>HHHHHHEFFADGKAGLELRNFYFNRDYRQPGASQSYSEEWAQGFLLRYESGYTEGLFGLGVDALGLLGVRLDSSPERSGSGLLPYSTSDRRAAHDYSSLGLTAKLRVSHSTLKIGTLMPRLPVVQFNDTRLHPQTFQGGLLEVNEIDGLALQFGQLRQVKQRDSTNAEDLGITRGNKRNVLAGRHPGSDRFDFAGGTYRWSERLSSSYHYA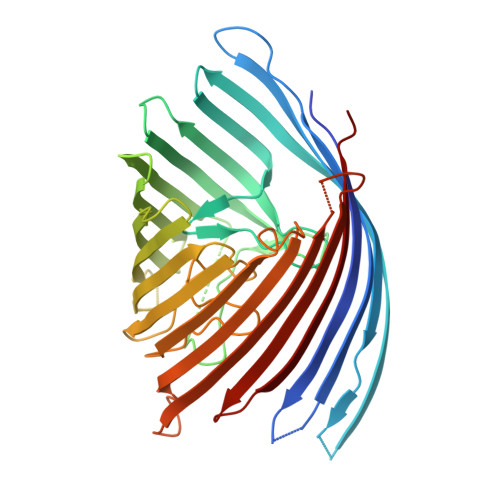NLEDFYRQHHLGVQHLLPLADDQSLKSDIRWARSTDEGGSRVNNRALNALFTYRLGGHAFGLGYQRMSGDSGFAYLAGTDPYLVNFVQIGDFANKDERSWQLRYDYDFAAIGLPGLTFMSRYLRGEHIDLLDGGGRGKEWERDTDIAYLVQSGPLKNLGIKLRNGTFRSDFGNDIDETRLIVSYALPLW[2x]>MSGSMKEEIKRLA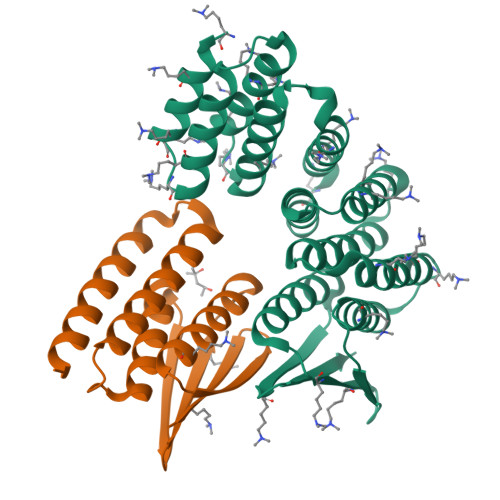EELKEKTKNEEIKRLAEEAAELAERSDDPEVLEVVKKALEEALKSKNEEKIELLLLVAVLVAEAGSVDAVEEKLEIALLALKLAEESKDPRIIRGALRAAIAALRSDDPLALKTVKEALERARASKDERLIRAILAAAYAFALLAVAGASAERLKEAEAIVKELIAAAEKGASPQELVLLVIEMMVKGMGVTMETHRSGNEVKVVIKGLHESQQEVLLEAVLFAAELMGVRVRIRFKGDTVTIVVREGSG[2x];>MSGEEAVRRRFEELLREALAFRERTGGRRETLEHAVRLARELAEFAASHPEFNRQEAVLLAIELMVRAMGVTMETHRSGNEVKVVIKGLNIDEQVALYRAVRETSKIMGVETEIEVEGDTQTIVVREGSG[2x]>GTAAGCAGCATC[3x];>AGCUUAC[3x];>GATGCTC[3x]

In this reversible process, a strand of RNA hybridizes to one strand of a DNA duplex while displacing the other strand, requiring concomitant disruption of DNA:DNA base pairs and formation of RNA:DNA base pairs. The defining feature of RNA/DNA strand exchange is the junction where the RNA:DNA helix abuts the DNA:DNA helix. While stacking in DNA-only junctions is thought to occur as it would in an uninterrupted B-form duplex, an analogous structural prediction cannot be made for RNA/DNA junctions because the two component helices are predisposed to different geometries: B-form for the DNA:DNA helix and a variant of A-form for the RNA:DNA helix. Here we present the X-ray crystal structure of an RNA-5′/DNA-3′ strand exchange junction, which undergoes an A-to-B transition without loss of base pairing or stacking across the exchange point.

Inspired by previous crystallographic studies of double-stranded DNA dodecamers, we designed crystallization constructs that contained a “template” DNA strand (12 nucleotides) and two “exchanging” RNA and DNA oligonucleotides that were complementary to each half of the template DNA strand. Only the flapped construct in the RNA-5′/DNA-3′ polarity yielded well-diffracting crystals (anisotropic resolution of 1.6 to 2.2 Å). In this structure, the asymmetric unit contains three molecules (a “molecule” comprises one DNA 12-mer and its complementary RNA and DNA 7-mers). Along one lattice direction, Molecules 1 and 2 form a continuous network of stacked helices, in which the external RNA:DNA duplex terminus of each Molecule 1 stacks on the equivalent terminus of Molecule 2, with a similar reciprocal interaction for the external DNA:DNA duplex termini (a “head-to-head” and “foot-to-foot” arrangement). Along another lattice direction, symmetry-related instances of Molecule 3 create a head-to-foot helical network. The three molecules of the asymmetric unit exhibit canonical Watson-Crick base pairing at all twelve nucleotides of the template DNA strand, and they are generally similar in conformation (RMSDMol1,Mol2 = 0.70 Å; RMSDMol1,Mol3 = 1.5 Å, RMSDMol2,Mol3 = 1.8 Å). Notably, the similarity of all three molecules at the three base pairs on either side of the exchange point (RMSDMol1,Mol2 = 0.57 Å; RMSDMol1,Mol3 = 0.50 Å, RMSDMol2,Mol3 = 0.75 Å) suggests that the conformation in this region represents a low-energy solution to the stacking of RNA:DNA and DNA:DNA helices. The structure reveals that the A-to-B helical transition involves a combination of helical axis misalignment, helical axis tilting and compression of the DNA strand within the RNA:DNA helix, where nucleotides exhibit a mixture of A- and B-form geometry. Notably, dramatic misalignment of the RNA:DNA/DNA:DNA helical centers is observed only in the present structure and is likely enabled by the break in the exchanging strands, which is not a feature of Okazaki fragments.>SNASVFDLFSIGIGPSSSHTVGPMLAANAFLQLLEQKNLFDKTQRVKVELYGSLALTGKGHGTDKAILNGLENKAPETVDPASMIPRMHEILDSNLLNLAGKKEIPFHEATDF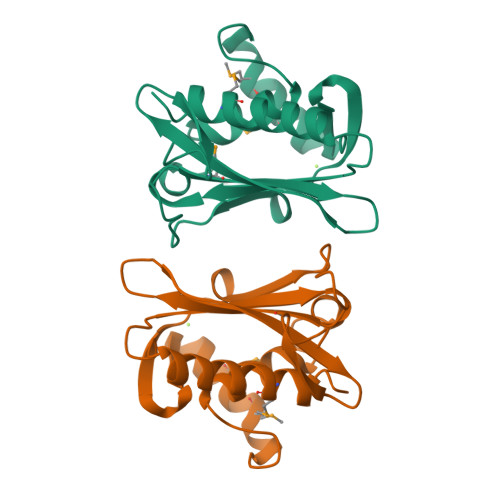LFLQKELLPKHSNGMRFSAFDGNANLLIEQVYYSIGGGFITTEEDFDK[2x]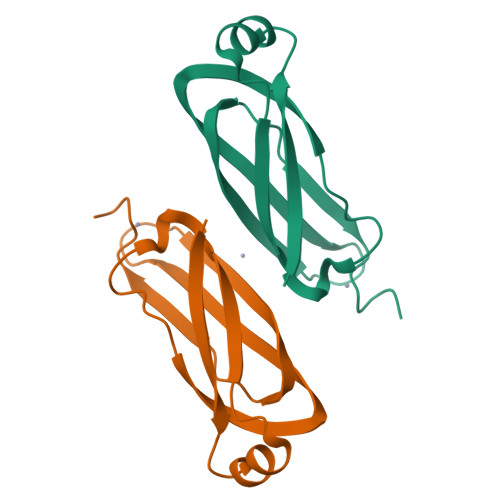>MTRLEVLIRPTEQTAAKANAVGYTHALTWVWHSQTWDVDSVRDPSLRADFNPEKVGWVSVSFACTQCTAHYYTSEQVKYFTNIPPVHFDVVCADCERSVQ[2x]> ETLRGCPTHCHCEPDGRMLLRVDCSDLGLSELPSNLSVFTSYLDLSMNNISQLLPNPLPSLRFLEELRLAGNALT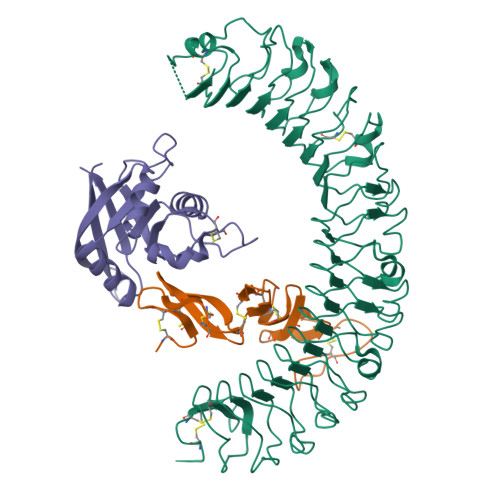YIPKGAFTGLYSLKVLMLQNNQLRHVPTEALQNLRSLQSLRLDANHISYVPPSCFSGLHSLRHLWLDDNALTEIPVQAFRSLSALQAMTLALNKIHHIPDYAFGNLSSLVVLHLHNNRIHSLGKKCFDGLHSLETLDLNYNNLDEFPTAIRTLSNLKELGFHSNNIRSIPEKAFVGNPSLITIHFYDNPIQFVGRSAFQHLPELRTLTLNGASQITEFPDLTGTANLESLTLTGAQISSLPQTVCNQLPNLQVLDLSYNLLEDLPSFSVCQKLQKIDLRHNEIYEIKVDTFQQLLSLRSLNLAWNKIAIIHPNAFSTLPSLIKLDLSSNLLSSFPITGLHGLTHLKLTGNHALQSLISSENFPELKVIEMPYAYQCCAFGVCENNGNNGDSVQCSPSGTHHHHHHHHHH;> ETGICKGCLSCSKDNGCSRCQQKLFFFLRREGMRQYGECLHSCPSGYYGHRAPDMNRCARCRIENCDSCFSKDFCTKCKVGFYLHRGRCFDECPDGFAPLDETMECVEGTHHHHHHHHHH;> ETGKETAFVEVVLFESSPSGDYTTHTTGLTGRFSRAGAMLSAEGEIVQMHPLGLCNNNDEEDLYEYGWVGVVKLEQPELDPKPCLTVLGKAKRAVQRGATAVIFDVSENPEAIDQLNQGSEDPLKRPVVYVKGADAIKLMNIVNKQKVARARIQHLGTKHHHHHH>[2x]GSGMLNRVEDILHELEGQVEPLKIQASIAKDYLEKKKELEHVEIALTAYDIEELHGKWSTLKEKVQMAKESGGSGGSTLLKDEEVKLGRMEVELDNLLQYLREEYSLSFEGAKEKYQLETDPEEARKRVKLIKLAIEELGTVNLGSIDEFERVNERYKFLSEQKEDL

Multi-subunit SMC complexes control chromosome superstructure and promote chromosome disjunction, conceivably by actively translocating along DNA double helices. SMC subunits comprise an ABC ATPase “head” and a “hinge” dimerization domain connected by a 49 nm coiled-coil “arm. The heads undergo ATP-dependent engagement and disengagement to drive SMC action on the chromosome. Here, we elucidate the architecture of prokaryotic Smc dimers by high-throughput cysteine cross-linking and crystallography.

Next, we solved the crystal structure of a head-proximal Smc segment, named BsSmcCC1, at a resolution of 1.9 Å. The top and bottom helices αC1 and αC4, respectively, form coiled-coil contacts with the top and bottom segment of αN1 in the BsSmcCC1 structure. Helix αC2 lies perpendicular to αN1 to connect helix αC1 with αC3, which is located on the opposite side of αN1. Helix αC3 makes a coiled-coil-like interaction with the middle part of αN1. A short loop joins αC3 to αC4 across αN1. Overall, BsSmcCC1 folds into a peculiar, elongated structure, where C-terminal sequences form three helix-loop repeats that spirally contact the continuous α helix αN1. We term the coiled-coil interruption “Smc joint,” as it connects two straight parts of the Smc protein at a slight angle. Crystal packing does not involve the formation of a “rod-like” dimer of BsSmcCC1. To establish how two BsSmcCC1 monomers might be arranged within the Smc dimer, we mapped cysteine cross-linking efficiencies onto the structure of BsSmcCC1. Importantly, almost all side chains of these residues point toward the same face of the elongated BsSmcCC1 structure as is expected for an element of a rod-shaped Smc dimer.> MIVKRPVSASLARAFFYIVLLSILSTGIALLTLASSLRDAEAINIAGSLSMQSYRLGYDLQSGSPQLNAHRQLFQQALHSPVLTNLNVWYVPEAVKTRYAHLNANWLEMNNRLSKGDLPWYQANINNYVNQIDLFVLALQHYAERKMLLVVAISLAGGIGIFTLVFFTLRR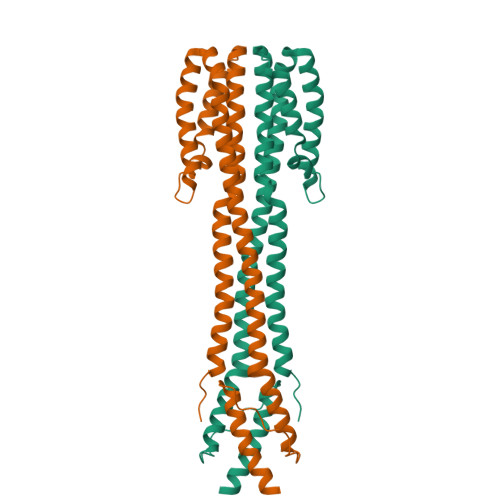IRHQVVAPLNQLVTASQRIEHGQFDSPPLDTNLPNELGLLAKTFNQMSSELHKLYRSLEHHHHHH> GCCGACGGGTTCACAGTCCGTCGGC

Cd2+-binding aptamers have been extensively utilized in the development of Cd2+-detecting devices; however, the underlying mechanisms remain elusive. This study reports four Cd2+-bound DNA aptamer structures, representing the only Cd2+-specific aptamer structures available to date. In all the structures, the Cd2+-binding loop (CBL-loop) adopts a compact, double-twisted conformation and the Cd2+ ion is mainly coordinated with the G9, C12 and G16 nucleotides. Other nucleotides of the loop and the G8–C18 pair of the stem also affect the Cd2+ binding, via proper folding and/or stabilizing the conformation of the CBL-loop.

Though we failed to obtain any crystal for DNA1 with either A13 or C14 mutated, one T22C variant structure in the presence of Cd2+ was successfully solved. The structure belongs to the P43212 space group and contains one T22C–Cd2+ complex per asymmetric unit. Packing of the T22C–Cd2+ complex in the crystal lattice is different from that in all other structures. Supplementary Figure S10B illustrates that each T22C–Cd2+ complex is surrounded by several T22C molecules; however, none of them interact with A13 or C14. Unlike all other structures, A13 does not interact with symmetry-related C14 in the T22C–Cd2+ complex structure; the conformation of the CBL-loop in the T22C–Cd2+ complex should be the closest to the one in solution. Compared to the native DNA1–Cd2+ structure, the nucleobase of A13 undergoes 40° rotation in the T22C–Cd2+ complex structure. The nucleobase of A13 stacks with T11 from the same CBL-loop, forming extensive hydrophobic interactions. Different from the native DNA1 and other variants, the nucleotide T22 was replaced by C22 in the T22C variant. In the T22C–Cd2+ complex structure, G4 and C22 formed one regular W–C pair. The KD values of the T22C variant and the native DNA1 are comparable.> SMTDQAFVTLTTNDAYAKGALVLGSSLKQHRTTRRLVVLATPQVSDSMRKVLETVFDEVIMVDVLDSGDSAHLTLMKRPELGVMLTKLHCWSLTQYSKCVFMDADTLVLANIDDLFDREELSAAPDPGWPDCFNSGVFVYQP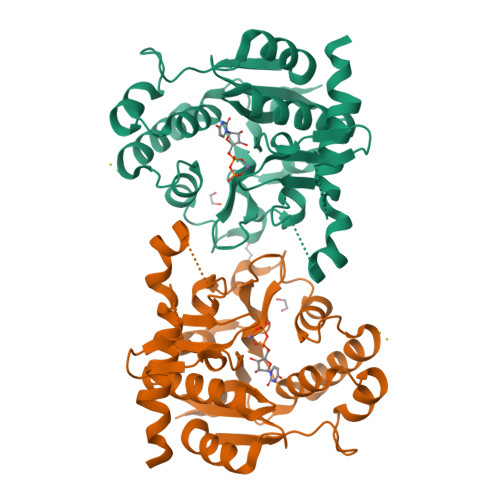SVETYNQLLHLASEQGSFDGGDQGILNTFFSSWATTDIRKHLPFIYNLSSISIYSYLPAFKVFGASAKVVHFLGRVKPWNYTYDPKTKSVKSEAHDPNMTHPEFLILWWNIFTTNVLPLLQ>MNLPDNSIHLQLPRPVCEAIIRPVPEHRADQELSEIYRDLKATFGVPWVGVITQAVAYYRPFFAEAWRRFAPSAKTHFFERASDDIRIRSWELMGQSFVIEGQTDRLREMGYSVREIGQIRAVLDIFDYGNPKYLIFATAIKEGLLSGRTFGGAAGDARCHFPRSPICQIDPIPVMVEEHHAGGTLSQVYADIKQTLQLPFINSDYKAMARWPSYLEQAWGALKPCIDTPAYQAG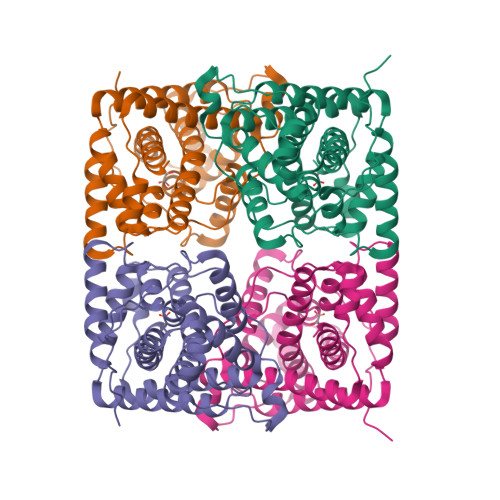RFDINARALAALDALPTAYRMSRDDALQAGLSEAQTDELIQVISLFQWMLSGLVLNVTHFKQQALK[4x]> SNADSLPERIDLFVSLFDYNSATTSYDIRSIQTDFP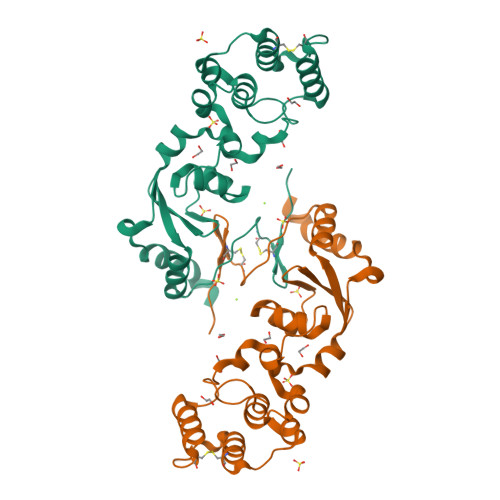TRLLTPDSMLPQTSEYPLKDIQLLYKLAQSCTGKLPLSPLITEPLVFTRSLCKGSSLSPRWFARSGLIHPGGGTYAFRYAEKYPAQFANLLPYMHIQERPNAAEGTLLYHLQNMGEDAINALVSGASMFGSGSDLWLRKGDIYYLFNEETWLTNANKAGLSYSLLSADCFIQRGNICWDVEDHS> MLQPVFTLKLRHKISPRMVAVGRYDGTHPCLAAATQAGKVFIHNPHSRSQHLGAPRVLQSPLESDVSLLNINQTVSCLTAGVLNPELGYDALLVGTQTNLLAYDVYNNSDLFYREVADGASAIVLGTLGDITSPLAIIGGNCALQGFNHEGNDLFWTVTGDNVHSLALCDFDGDGKKELLVGSEDFDIRVFKEDEIVAEMSETEIITSLCPMYGSRFGYALSNGTVGVYDKTARYWRIKSKNQAMSIHAFDLNSDGVCELITGWSNGKVDARSDRTGEVIFKDNFSSAIAGVVEGDYRMEGCQQLICCSVDGEIRGYLPGTAEMRGNLMDISVEQDLIRELSQKKQNLLLELRNYEENAKAELSSPLNEADGHRGVIPANTKHHTALSVSLGSEAQAAHAELCISTSNDTIIRAVLIFAEGVFAGESHVVHPSVHHLSSSVRIPITPPKDIPVDLHLKTFVGYRSSTQFHVFELTRQLPRFSMYALTSPDPASEPLSYVNFIIAERAQRVVMWLNQNFLLPEDTNIQNAPFQVCFTSLRNGGQLYIKIKLSGEITVNTDDIDLAGDIIQSMASFFAIEDLQVEADFPVYFEELRKVLVKVDEYHSVHQKLSADMADNSNLIRSLLVQAEDARLMRDMKTMKNRYKELYDLNKDLLNGYKIRCNNHTELLGSLKAVNQAIQRAGHLRVGKPKNQVITACRDAIRSNNINMLFRIMRVGTASS;> MDLNLNRADYLQVGVTSQKTMKLLPASKHRATQKVVVGDHDGIVMCFGMKKGEAVTVFKTLPGQKIARLELGGALNTPQEKIFIAAGSEIRGFTKRGKQFLSFETNLTESIKAMHISGSDLFLSASYIYNHYCDCKDQHYYLSGDKINDVICLPVERLLREVPVLACQDRVLRVLQGSDVTYEIEVPGPPTVLALHNGNGGDSGEDLLFGTSDGKLGLIQITTSKPIHKWEIRNEKKRGGILCVDSFDIVGDGVKDLLVGRDDGMVEVYGFDNANEPVLRFDHTLSESVTSIQGGCVGKDGYDEIVVSTYSGWITGLTTEPVHKESGPGEELKFNQEMQNKISSLRSELEQLQYKVLQEREKYQQSSQSSKAKSAVPSFSVNDKFTLNKDDASYSLILEVQTAIDNVLIQSDVPIDLLDVDKNSAVVSFSSCDSESNDNFLLATYRCQANTTRLELKIRSIEGQYGTLQAYVTPRIQPKTCQVRQYHIKPLSLHQRTHFIDHDRPMNTLTLTGQFSFSELHSWVVFCMPEVPEKPPAGECVTFYFQNTFLDTQLESTYRKGEGVFKSDNISTISILKDVLSKEATKRKINLNISYEINEVSVKHTLKLIHPKLEYQLLLAKKVQLIDALKELQVHEGNTNFLIPEYRCILEEADHLQEEYKKQPAHLERLYGMITDLFIDKFKFKGTNVKTKVPLLLEILDSYDQNALIAFFDAA;> MAATSSSDSDGGKGESEANSKWLDSLSDSMANIHTFSACLALADFHGDGEYKLAMGDLGPDGRQPRLKVLKGHTLVSQKPLPDLPAAAVTFLMASHEPRTPALAIASGPCVYVYKNLKPYFKFSLPSLPTNPLEQDLWNQAKEDQIDPLTLKEMLEGIREKAEVPLSVQSLRFLPLELSEMEAFVNQHKSKSIRRQTVITTMTTLKKNLADEDAVSCLVLGTENKELLVLDPEAFTILAKMSLPSVPAFLEASGQFDVEFRLAAACRNGSIYILRRDSKRPKYCIELGAQPVGLVGVHKVLVVGSNQDSLHGFTYKGKRLWTVQMPAAILAMNLLEQHSRGLQAVMAALANEEVRIYHDKVLLNVIRTPEAVTSLCFGRYGREDNTLIMTTLGGGLIIKILKRTAVFAEGGGEAGPPPSQAIKLNVPRKTRLYVDQTLREREAGTAMHRTFQADLYLLRLRAARAYVQALESSLSPVSLTAREPLKLHAVVQGLGPTFKLTLHLQNTSTARPILGLVVCFLYNEVLYALPRAFFKVPLLVPGLNYPLETFVKSLSDKGISDIIKVLVLREGQSTPLLSAHINMPMSEGLAAD;> MAEEKLSARTQLPVSAESQKPVLKKAPEFPILEKQNWLIHLYYIQKDYEACKAVIKEQLQETHGLCEYAIYVQALIFRLEGNIQESLRLFQMCAFLSPQCADNLKQVARSLFLLGKHKAAIEVYNEAAKLNQKDWEICHNLGVCYIYLKQFDKAQDQLHNALHLNRHDLTYIMLGKIFLLKGDLDKAIEIYKKAVEFSPENTELLTTLGLLYLQLGIYQKAFEHLGNTLTYDPTNYKAILAAGSMMQTHGDFDVALTKYKVVACAVIESPPLWNNIGMCFFGKKKYVAAISCLKRANYLAPLDWKILYNLGLVHLTMQQYASAFHFLSAAINFQPKMGELYMLLAVALTNLEDSENAKRAYEEAVRLDKCNPLVNLNYAVLLYNQGEKRDALAQYQEMEKKVNLLKYSSSLEFDPEMVEVAQKLGAALQVGEALVWTKPVKDPKSKHQTASTSKAAGFQQPLGSNQALGQAMSSAATCRKLSSGAGGTSQLTKPPSLPLEPEPTVEAQPTEASAQTREK;> MEPLLLAWSYFRRRRFQLCADLCTQMLEKSPCDQAAWILKARALTEMVYVDEIDVDEEGIAEMILDENAIAQVPRPGTSLKLPGTNQTGGPSPAVRPVTQAGRPITGFLRPSTQSGRPGTIEQAIKTPRTAYTARPIASSSGRFVRLGTASMLTSPDGPFINLSRLNLAKYAQKPKLAKALFEYIFHHENDVKTALDLAALSTEHSQYKDWWWKVQIGKCYYRLGLYREAEKQFKSALKQQEMVDTFLYLAKVYISLDQPLTALNLFKQGLDKFPGEVTLLCGIARIYEEMNNISSATEYYKEVLKQDNTHVEAIACIGSNHFYTDQPEVALRFYRRLLQMGVYNCQLFNNLGLCCFYAQQYDMTLTSFERALSLAENEEEVADVWYNLGHVAVGTGDTNLAHQCFRLALVSNNQHAEAYNNLAVLEMRRGHVEQAKALLQTASSLAPHMYEPHFNFATISDKIGDLQRSYAAAKKSEAAFPDHVDTQHLIKQLEQHFAML;> MSVLDALWEDRDVRFDVSSQQMKTRPGEVLIDCLDSVEDTKGNNGDRGRLLVTNLRIVWHSLALPRVNLSIGYNCILNITTRTANSKLRGQTEALYVLTKCNSTRFEFIFTNLVPGSPRLYTSLIAVHRAYETSKMYRDFKLRSALIQNKQLRLLPQENVYNKINGVWNLSSDQGNLGTFFITNVRIVWHANMNDSFNVSIPYLQIRSVKIRDSKFGLALVIESSQQSGGYVLGFKIDPVEKLQESVKEINSLHKVYSANPIFGVDYEMEEKPQPLEALTVKQIQDDVEIDSDDHTDAFVAYFADGNKQQDREPVFSEELGLAIEKLKDGFTLQGLWEVMN;> MAETKSMFREVLPKQGQLYVEDITTMVLCKPKLLPLKSLTLEKLEKMQQAAQDTIHQQEMTEKEQKITH;> MSLFKARDWWSTVLGDKEEFDQGCLCLADVDNTGNGQDKIIVGSFMGYLRIFNPHPVKTGDGAQAEDLLLEVHLRDPILQVEVGKFVSGTEMLHLAVLHSRKLCVYSVSGTLGNVEHGNQYQIKLMYEHNLQRTACNMTYGSFGGVKGRDLICIQSVDGMLMVFEQESYAFGRFLPGSLLPGPLAYSSRTDSFITVSSCHQVESYKYQVLAFATDADKRQETEQQKHGSGKRLVVDWTLNIGEQAIDICIVSFIQSASSVFVLGERNFFCLKDNGQIQFMKKLDYSPSCFLPYCSVSEGTINTLIGNHNNMLHIYQDVTLKWATQLPHVPVAVRVGCLHDLKGVIVTLSDDGHLQCSYLGTDPSLFQAPKVESRELNYDELDMELKELQKVIKNVNKSQDVWPLTEREDDLKVSAMVSPNFDSVSQATDVEVGADLVPSVTVKVTLKNRVALQKIKLSIYVQPPLVLTGDQFTFEFMAPEMTRTVGFSVYLKGSYSPPELEGNAVVSYSRPTERNPDGIPRVSQCKFRLPLKLVCLPGQPSKTASHKLTIDTNKSPVSLLSLFPGFAKQSEDDQVNVMGFRFLGGSQVTLLASKTSQRYRIQSEQFEDLWLITNELIIRLQEYFEKQGIKDFTCSFSGSVPLEEYFELIDHHFELRINGEKLEELLSERAVQFRAIQRRLLTRFKDKTPAPLQHLDTLLDGTYKQVIALADAVEENQDNLFQSFTRLKSATHLVILLIGLWQKLSADQIAILEAAFLPLQQDTQELGWEETVDAALSHLLKTCLSKSSKEQALNLNSQLGIPKDTSQLKKHITLFCDRLAKGGRLCLSTDAAAPQTMVMPGGCATIPESDLEGRSIDQDSSELFTNHKHLMVETPVPEVSPLQGVTE

Patched 1, GPR161, SMO and other ciliary membrane proteins are all ferried out of cilia in a regulated manner by an evolutionarily conserved complex of eight Bardet-Biedl Syndrome (BBS) proteins, the BBSome. Our recent cryo-electron microscopy (cryo-EM) structure of the BBSome revealed that the BBSome exists mostly in an auto-inhibited, closed conformation in solution and undergoes a conformational change as it is recruited to membranes by ARL6GTP. Given that ARL6GTP triggers polymerization of a membrane-apposed BBSome/ARL6 coat and enables BBSome-mediated TZ crossing, the ARL6GTP-bound BBSome conformation represents the active form of the complex. Here we determine high-resolution structures of the BBSome alone and bound to ARL6GTP, and we map the BBSome–SMO interaction to model how the membrane-associated BBSome–ARL6GTP complex recognizes its cargoes.

Following on our previous strategy, we purified the BBSome to near-homogeneity from retinal extract and analyzed its structure by single-particle cryo-EM. The advent of higher throughput direct detector cameras and faster automated data-collection procedures combined with improvements in data processing with new tools implemented in RELION-3 led to a BBSome map at an overall resolution of 3.4 Å from an initial dataset of 770,345 particles. The BBSome is composed of 29 distinct domains characteristic of sorting complexes. α-solenoids, β-propellers, pleckstrin homology (PH) and appendage domains are all present in multiple copies and our previous map made it possible to build a Cα backbone model that encompassed 25 out of 29 domains (PDB-Dev accession PDBDEV_00000018; Chou et al., 2019). For building the current model, the previous Cα model was docked into the map, and the higher-resolution map enabled us to confidently assign side chains for most regions. The new map allowed us to build the coiled-coil domains of BBS1 and BBS9, for which densities were not well-defined in the previous map. Altogether, 27 out of 29 domains distributed across the 8 BBSome subunits could be modeled. Despite the increased resolution of the current density map, the gamma-adaptin ear (GAE) domains of BBS2 and BBS7 could not be modeled, and side chains could not be assigned for BBS2βprop, BBS2cc, BBS7βprop and BBS7cc. Consistent with our previous observations based on a 4.9 Å resolution map of the BBSome, the new BBSome structure cannot accommodate binding to ARL6GTP. Fitting a homology model of the bovine BBS1βprop–ARL6GTP complex (based on the X-ray structure of the Chlamydomonas complex; Mourão et al., 2014) in either BBSome structure caused a steric clash between ARL6GTP and a region encompassing BBS2βprop and BBS7cc. These data support a model in which the BBSome exists in an autoinhibited form in solution and undergoes a conformational opening upon recruitment to membranes by ARL6GTP, similar to other sorting complexes such as COPI, AP-1 and AP-2.BTB (bric-a-brack, Tramtrack, and broad complex) is a diverse group of protein-protein interaction domains found within metazoan proteins. The Tramtrack group (TTK) is a distinct type of BTB domain, which can multimerize. TTK-type BTB domains contain a highly conserved N-terminal FxLRWN motif, where x is a hydrophilic residue. Thus, the TTK-type BTB domains are a structurally and functionally distinct group of protein domains specific to Arthropodan transcription factors.

To enhance particle contrast on cryo-EM images, we used the BTB domain of CG67651-133 fused to MBP (40 kDa), which resulted in a monomer Mw of 56 kDa. Iterative masked refinement excluding flexible MBP regions resulted in a final reconstruction of core CG67651-133 multimer at a resolution of 3.3 Å (full data processing flowchart is shown at Figure 3—figure supplement 1). The map clearly shows the hexameric assembly consisting of three dimers. CG6765 hexamer consists of three canonical BTB dimers with extensive hydrophobic molecular contacts and main-chain hydrogen bonds (N78, V82, Y84, V86) forming a β-sheet between two parallel β4-strands (corresponding to B3 according to Stogios et al., 2005). In addition, a bifurcated hydrogen bond is formed from the side chain hydroxy group of Y84 of one dimer to the sidechain of T77 and main-chains of either N78 or I76 of the second dimer. Furthermore, a few inter-dimer hydrogen bonds are formed between (i) T50 and T73, (ii) N78 and N80, and (iii) side chain hydroxy group of Y36 and P75/M70 main chain atoms. Interdimeric interactions were further strengthened by hydrophobic contacts between A2 (F66, M70, P75), the loop preceding B1 (I48), and B2/B1/B3 sheet (V34, V86), with the B3 strand formed by residues highly conserved only within the TTK group. Residues with large hydrophobic or aromatic side-chains at positions corresponding to Y84 and V86 of CG6765 are characteristic for all TTK-type BTBs, whereas residues involved in stabilizing interactions at B1/A2 and adjacent loops are less conserved. The N-terminal TTK-motif is located within the first β-strand and is involved only in intra-dimer stabilization forming antiparallel beta-sheet with B4. Central part of the hexamer forms a pore, residues of loop regions surrounding the pore are not conserved, thus it is unlikely that it can possess some physiological function.

>AENYHLKWDSHLTYLNSSIATLYKNEKFADVVLYSSYNSSGIPSDIPTVGISAHKFILSASSQFFATMFETAPITNPNGVLYVVLPPDLSHRAIQILVQYMYSGEATVSNDILNEVLRGGEILKIRGLCRT[6x]>[2x]MVLDNLGKALANTLKKIAR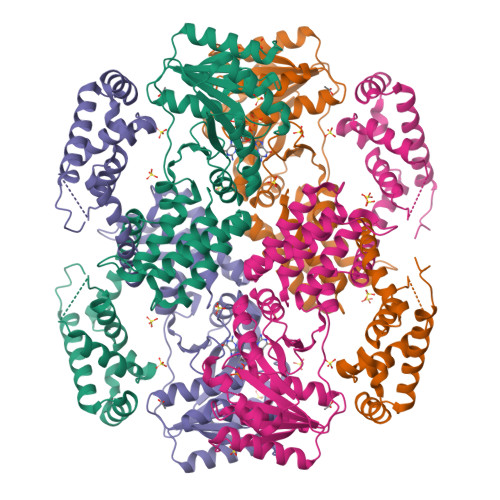ASSVDEALIKELVRDIQRALIQADVNVRLVLQLTREIQRRALEEKPPAGISKKEHIIKIVYEELTKFLGTEAKPIEIKEKPTILLMVGIQGSGKTTTVAKLARYFQKRGYKVGVVCSDTWRPGAYHQLRQLLDRYHIEVFGNPQEKDAIKLAKEGVDYFKSKGVDIIIVDTAGRHKEDKALIEEMKQISNVIHPHEVILVIDGTIGQQAYNQALAFKEATPIGSIIVTKLDGSAKGGGALSAVAATGAPIKFIGTGEKIDDIEPFDPPRFVSRLLGLGDIQGLLEKFKELEKEVEIKEEDIERFLRGKFTLKDMYAQLEAMRKMGPLKQILRMIPGLGYSLPDDVISIGEERLKKFKVIMDSMTEEELLNPEIINYSRIKRIARGSGTSTKDVKELLDQYRQMKKLFKSMNKRQLSRLARRFGM> SNLNPNAPEFHPGVPWKG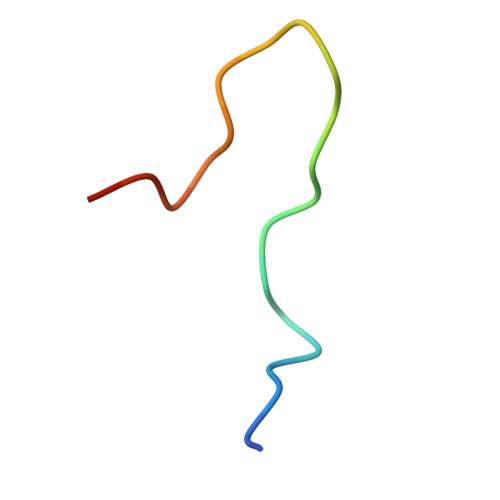LQNI>LYPEEILDTHWELWKKTHRKQYNNKVDEISRRLIWEKNLKYISIHNLEASLGVHTYELAMNHLGDMTSEEVVQKMTGLKVPLSHSRSNDTLYIPEWEGRAPDSVDYRKKGYVTPVKNQGQCGSCWAFSSVGALEGQLKKKTGKLLNLSPQNLVDCVSENDGCGGGY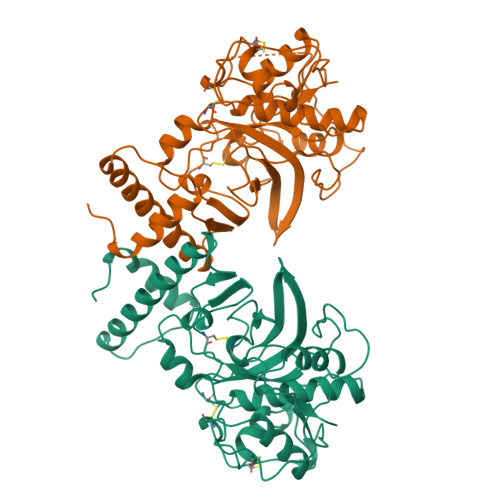MTNAFQYVQKNRGIDSEDAYPYVGQEESCMYNPTGKAAKCRGYREIPEGNEKALKRAVARVGPVSVAIDASLTSFQFYSKGVYYDESCNSDNLNHAVLAVGYGIQKGNKHWIIKNSWGENWGNKGYILMARNKNNACGIANLASFPKM[4x]>MEQSRSQQRGGEQSWWGSDPQYQYMPFEHCTSYGLPSENGGLQHRLRKDAGPRHNVHPTQIYGHHKEQFSDREQDIGMPKKTGSSSTVDSKDEDHYSKCQDCIHRLGQVVRRKLGEDGIFLVLLGLLMALVSWSMDYVSAKSLQAYKWSYAQMQPSLPLQFLVWVTFPLVLILFSALFCHLISPQAVGSGIPEMKTILRGVVLKEYLTMKAFVAKVVALTAGLGSGIPVGKEGPFVHIASICAAVLSKFMSVFCGVYEQPYYYSDILTVGCAVGVGCCFGTPLGGVLFSIEVTSTYFAVRNYWRGFFAATFSAFVFRVLAVWNKDAVTITALFRTNFRMDFPFDLKELPAFAAIGICCGLLGAVFVYLHRQVMLGVRKHKALSQFLAKHRLLYPGIVTFVIASFTFPPGMGQFMAGELMPREAISTLFDNNTWVKHAGDPESLGQSAVWIHPRVNVVIIIFLFFVMKFWMSIVATTMPIPCGGFMPVFVLGAAFGRLVGEIMAMLFPDGILFDDIIYKILPGGYAVIGAAALTGAVSHTVSTAVICFELTGQIAHILPMMVAVILANMVAQSLQPSLYDSIIQVKKLPYLPDLGWNQLSKYTIFVEDIMVRDVKFVSASYTYGELRTLLQTTTVKTLPLVDSKDSMILLGSVERSELQALLQRHLCPERRLRAAQEMARKLSELPYDGKARLAGEGLPGAPPGRPESFAFVDEDEDEDLSGKSELPPSLALHPSTTAPLSPEEPNGPLPGHKQQPEAPEPAGQRPSIFQSLLHCLLGRARPTKKKTTQDSTDLVDNMSPEEIEAWEQEQLSQPVCFDSCCIDQSPFQLVE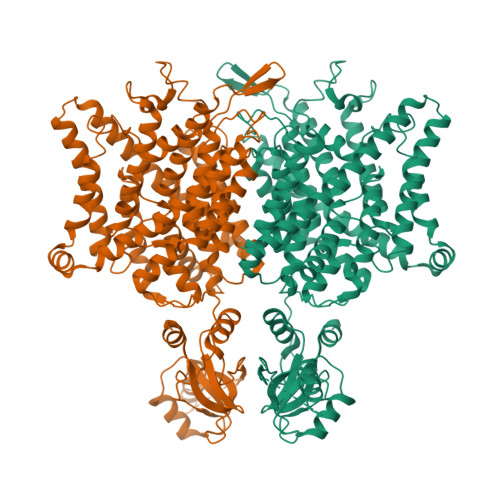QTTLHKTHTLFSLLGLHLAYVTSMGKLRGVLALEELQKAIEGHTKSGVQLRPPLASFRNTTSTRKSTGAPPSSAENWNLPEDRPGATGTGDVIAASPETPVPSPSPEPPLSLAPGKVEGELEELELVESPGLEEELADILQGPSLRSTDEEDEDELIL[2x]> HKILHRLLQ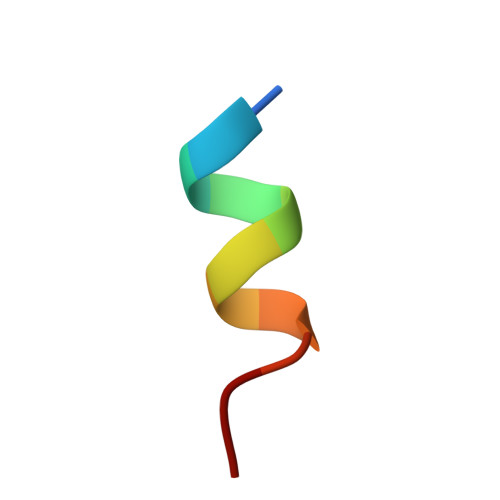DS>KREAEAKVRWPDFNQEAYVGGTMVRSGQDPYARNKSNQVESDKLRMDRAIPDTRHDQCQRKQWRVDLPATSVVITFHNEARSALLRTVVSVLKKSPPHLIKEIILVDDYSNDPEDGALLGKIEKVRVLRNDRREGLMRSRVRGADAAQAKVLTFLDSHCECNEHWLEPLLERVAEDRTRVVSPIIDVINMDNFQYVGASADLKGGFDWNLVFKWDYMTPEQRRSRQGNPVAPIKTPMIAGGLFVMDKFYFEELGKYDMMMDVWGGENLEISFRVWQCGGSLEIIPCSRVGHVFRKQHPYTFPGGSGTVFARNTRRAAEVWMDEYKNFYYAAVPSARNVPYGNIQSRLELRKKLSCKPFKWYLENVYPELRVPDHQDIAFGALQQGTNCLDTLGHFADGVVGVYECHNAGGNQEWALTKEKSVKHMDLCLTVVDRAPGSLIKLQGCRENDSRQ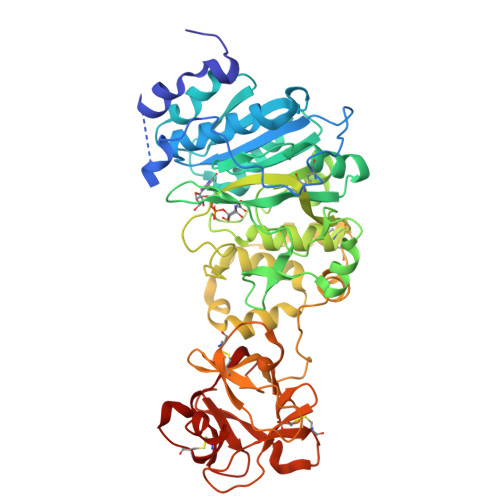KWEQIEGNSKLRHVGSNLCLDSRTAKSGGLSVEVCGPALSQQWKFTLNLQQ[2x]> MAEGEITTFTALTEKFNLPPGNYKKPKLLYCSNGGHFLRILPDGTVDGTRDRSDQHIQLQLSAESVGEVYIKSTETGQYLAMDTDGLLYGSQTPNEECLFLERLEENHYNTYISKKHAEKNWFVGLKKNGSCKRGPRTHYGQKAILFLPLPVSSD;> MAEDFVSENSNNKRAPYWTNTEKMEKRLHA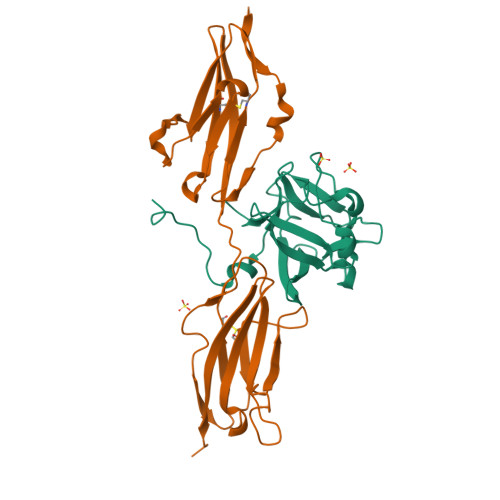VPAANTVKFRCPAGGNPMPTMRWLKNGKEFKQEHRIGGYKVRNQHWSLIMESVVPSDKGNYTCVVENEYGSINHTYHLDVVERSRHRPILQAGLPANASTVVGGDVEFVCKVYSDAQPHIQWIKHVEKNGSKYGPDGLPYLKVLKHSGINSSNAEVLALFNVTEADAGEYICKVSNYIGQANQSAWLTVLPKQQAPGREKE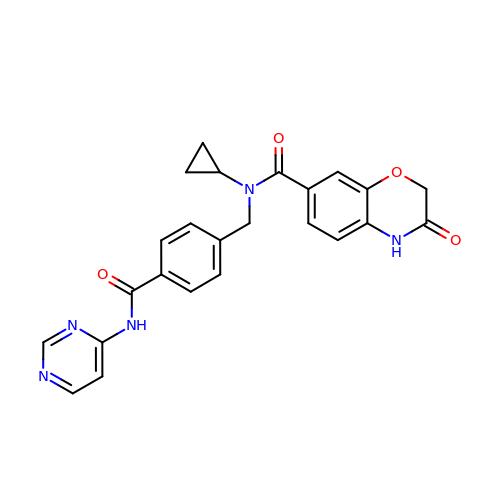N-cyclopropyl-3-oxo-N-({4-[(pyrimidin-4-yl)carbamoyl]phenyl}methyl)-3,4-dihydro-2H-1,4-benzoxazine-7-carboxamide | C24 H21 N5 O4 | KOZGEDUWAQFVAV-UHFFFAOYSA-N>[2x]GSMDPLSPPLCTLPPGPEPPRFVCYCEGEESGEGDRGGFNLYVTDAAELWSTCFTPDSLAALKARFGLSAAEDITPRFRAACEQQAVALTLQEDRA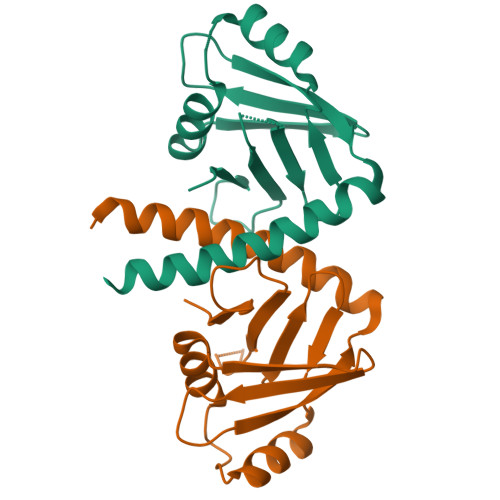SLTLSGGPSALAFDLSKVPGPEAAPRLRALTLGLAKRVWSLERRLAAAEETAVSPRKSPRPAGPQLFLPDPDPQRGGPGPGVRRRCPGESLINPGFKSKKPAGGVDFDET>GIDPFTNTKWDYKNKENGPHRWDKLHKDFEVCKSGKSQSPINIEHYYHTQDKADLQFKYAASKPKAVFFTHHTLKASFEPTNHINYRGHDYVLDNVHFHAPMEFLINNKTRPLSAHFVHKDAKGRLLVLAIGFEEGKENPNLDPILEGIQKKQNFKEVALDAFLPKSINYYHFNGSLTAPPCTEGVAWFVIEEPLEVSAKQLAEIKKRMKNSPNQRPVQPDYNTVIIKSSAETR[8x]

Bacterial carbonic anhydrases (CAs, EC 4.2.1.1), metalloenzymes that catalyse the hydration of carbon dioxide to bicarbonate and hydrogen ions, are emerging as new potential drug candidates due to their role in the survival, invasion and pathogenicity of bacteria. H. pylori has two different CAs, α-class and β-class (HpαCA and HpβCA). Here, we report structural analyses correlated with inhibition data, on complexes of HpαCA with AAZ and MZA. The structure reveals a fold characteristic of other αCAs of the known structure which contains a central 10-stranded, twisted β-sheet flanked by helices α1 and α2 on one side and α3–α5 on the other.

In both structures, the N atom of the sulfonamide moiety of the inhibitor acts as the fourth ligand in the tetrahedral coordination sphere for the zinc ion. The O1 atom of the sulfonamide group forms a hydrogen bond with the main-chain amide of Thr191. The sulfonamide group of AAZ is further stabilised by van der Waals contacts with the side chains of Val141 and Trp201. The thiadiazole moiety of AAZ stacks against the hydrophobic side of the cone-shaped surface leading into the active site and makes van der Waals contacts with Val131, Leu190 and Ala192. The AAZ molecule is further stabilised through a hydrogen bond between the O3 atom of its acetamido group and the Nδ atom of Asn108 (3.1 Å) and van der Vaals contact with the side chain of Lys88. Structural superimpositions showed that the positions of the AAZ molecule and the zinc ion are very similar in all eight subunits in the asymmetric unit. Superposition of the structures of the HpαCA/AAZ, SspCA/AAZ, TaCA/AAZ and HCAII/AAZ complexes shows a very good overlap of the zinc-coordinating sulfonamide moieties and only subtle differences in the orientation of the AAZ molecule, consistent with the absolute conservation of the protein residues that are important for AAZ recognition. In addition, examination of the superposition of the HpαCA/AAZ complex with the structures of free and substrate (CO2)-bound HCAII reveals that two sulfonamide oxygen atoms of AAZ are positioned close to the putative location of the oxygens of the CO2 substrate in the Michaelis complex (0.8 Å and 0.4 Å). Furthermore, in this superimposition the zinc-coordinating sulfonamide nitrogen occupies the position of the catalytic water/hydroxide ion Wat263. Thus, our analysis suggests that AAZ acts as a site-directed inhibitor by mimicking the catalytic transition state of the CO2 hydration reaction, which is in agreement with the tight binding reported for this inhibitor (Ki = 21 nM).> MAKEVVEVLVTGGRATAGPPL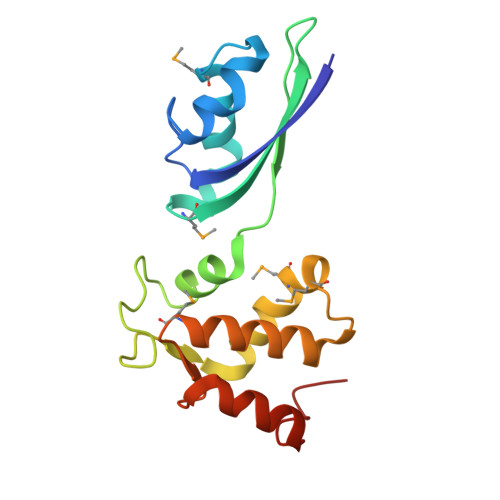GPAIGPLGVNVMQVVKEINEKTKDYEGMQVPVKVIVDTETRKFEIEVGIPPTTALIKKELGIETAAHEPRHEVVGNLTLEQVIKIAKMKKDAMLSYTLKNAVKEVLGTCGSMGVTVEGKDPKEVQKEIDAGVYDEYFKEE> GNVDLVFLFDGSMSLQPDEF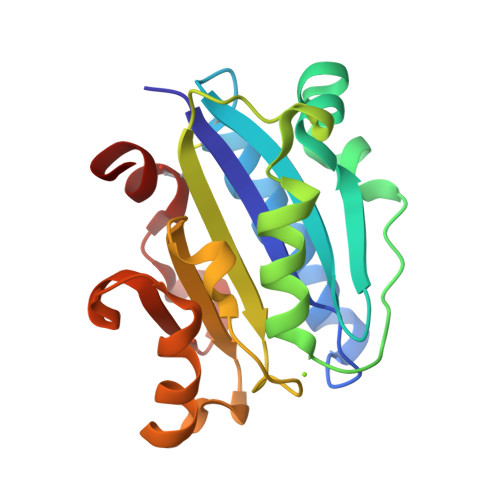QKILDFMKDVMKKCSNTSYQFAAVQFSTSYKTEFDFSDYVKRKDPDALLKHVKHMLLLTNTFGAINYVATEVFREELGARPDATKVLIIITDGEATDSGNIDAAKDIIRYIIGIGKHFQTKESQETLHKFASKPASEFVKILDTFEKLKDLCTELQKKI>[2x]GEFMVSIMLLKVEDLHVYRGNREILKGVNLTVEENEIHAIIGPNGAGKSTLAYTIMGISGYKPTKGRIIFKGVDIIDKNITERARMGMTLAWQEPARFEGIKVKNYLMLGMNEKYKKDKEIAEEKIREALKLVNLDPDKYLDRYVDETLSGGERKRIELASIICMEPDLAILDEPDSGIDIVSFDEIKRVFDYLKDKGCSLLVITHREELAEHADRVSLICAGEVIKSGDPK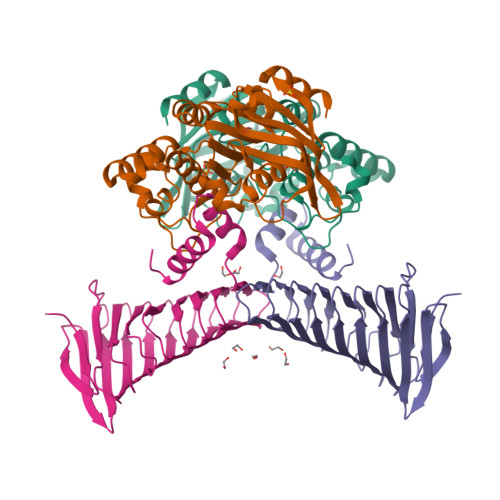EVGEFYKKECGKCYKKVPDGK;>[2x]GEFELMSIKEELMEIIEAIKYTSEKPEEIVHGKGPRIIVKESRIIDVQGDEGIILEGKEEDGKIKAKIIVKKGYKFKYPIHMCFGITEENISQIIDVEIILEEDSSISLMSHCSFPKGKGIKHIMNGIIKIGKNAKFSYNEFHYHGMDGDILVKPTVKVEIDEGGIYISNFTLTKGRIGTLDIEQEIIAKKDAIIDITTRTYAIKEDVVKVNEVVKLNGENAKCIIKSRGAAMDNSKISLKLKIEGNAPYSKGHIDCAEIVKGNAEVESIPIVVVRDDKARITHEAAIGSVDKKQLETLMAKGLDEDEATEIIVKGMIGDL>[8x]GASDPCAASEVARTVGSVAKSMGDYLDSHPETNQVMTAVLQQQVGPGSVA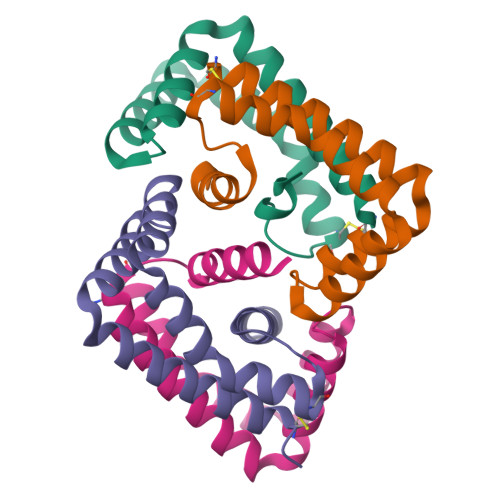SLKAHFEANPKVASDLHALSQPLTDLSTRCSLPISGLQAIGLMQAVQGARR> MAGQTTVDSRRQPPEEVDVLVVGAGFSGLYALYRLR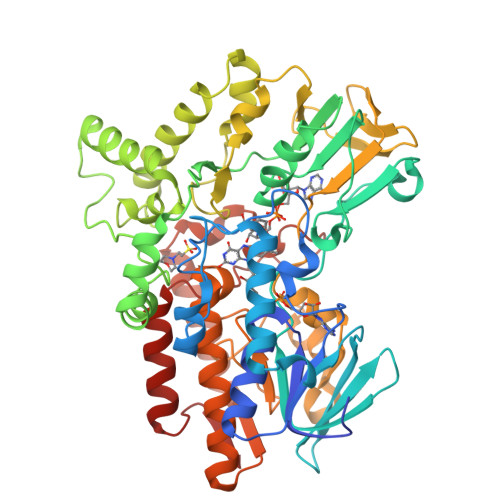ELGRSVHVIETAGDVGGVWYWNRYPGARCAIESIEYCYSFSEEVLQEWNWTERYASQPEILRYINFVADKFDLRSGITFHTTVTAAAFDEATNTWTVDTNHGDRIRARYLIMASGQLSVPQLPNFPGLKDFAGNLYHTGNWPHEPVDFSGQRVGVIGTGSSGIQVSPQIAKQAAELFVFQRTPHFAVPARNAPLDPEFLADLKKRYAEFREESRNTPGGTHRYQGPKSALEVSDEELVETLERYWQEGGPDILAAYRDILRDRDANERVAEFIRNKIRNTVRDPEVAERLVPKGYPFGTKRLILEIDYYEMFNRDNVHLVDTLSAPIETITPRGVRTSEREYELDSLVLATGFDALTGALFKIDIRGVGNVALKEKWAAGPRTYLGLSTAGFPNLFFIAGPGSPSALSNMLVSIEQHVEWVTDHIAYMFKNGLTRSEAVLEKEDEWVEHVNEIADETLYPMTASWYTGANVPGKPRVFMLYVGGFHRYRQICDEVAAKGYEGFVLT> KPGKCPVTYGQCLMLNPPNFCEMD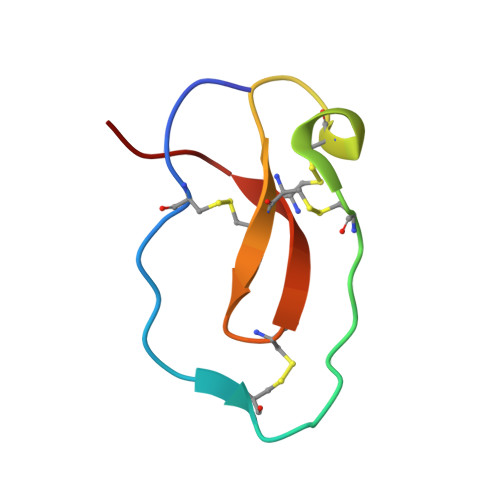GQCKRDLKCCMGMCGKSCVSPVK> MGGSEVGTVPVTWRLGVDVGERSIGLAAVSYEEDKPKEILAAVSWIHDGGVGDERSGASRLALRGMARRARRLRRFRRARLRDLDMLLSELGWTPLPDKNVSPVDAWLARKRLAEEYVVDETERRRLLGYAVSHMARHRGWRNPWTTIKDLKNLPQPSDSWERTRESLEARYSVSLEPGTVGQWAGYLLQRAPGIRLNPTQQSAGRRAELSNATAFETRLRQEDVLWELRCIADVQGLPEDVVSNVIDAVFCQKRPSVPAERIGRDPLDPSQLRASRACLEFQEYRIVAAVANLRIRDGSGSRPLSLEERNAVIEALLAQTERSLTWSDIALEILKLPNESDLTSVPEEDGPSSLAYSQFAPFDETSARIAEFIAKNRRKIPTFAQWWQEQDRTSRSDLVAALADNSIAGEEEQELLVHLPDAELEALEGLALPSGRVAYSRLTLSGLTRVMRDDGVDVHNARKTCFGVDDNWRPPLPALHEATGHPVVDRNLAILRKFLSSATMRWGPPQSIVVELGGGSAGGYAAVALRDRLLSYGEKNGVAQVAVFRGGVTAEARRWLDISIERLFSRVAIFAQSTSTKRLDRRHHAVDAVVLTTLTPGVAKTLADARSRRVSAEFWRRPSDVNRHSTEEPQSPAYRQWKESCSGLGDLLISTAARDSIAVAAPLRLRPTGALHEETLRAFSEHTVGAAWKGAELRRIVEPEVYAAFLALTDPGGRFLKVSPSEDVLPADENRHIVLSDRVLGPRDRVKLFPDDRGSIRVRGGAAYIASFHHARVFRWGSSHSPSFALLRVSLADLAVAGLLRDGVDVFTAELPPWTPAWRYASIALVKAVESGDAKQVGWLVPGDELDFGPEGVTTAAGDLSMFLKYFPERHWVVTGFEDDKRINLKPAFLSAEQAEVLRTERSDRPDTLTEAGEILAQFFPRCWRATVAKVLCHPGLTVIRRTALGQPRWRRGHLPYSWRPWSADPWSGGTPHHHHHH

Here we further characterized the PAM recognized by AceCas9 and report crystal structures of AceCas9 without its HNH domain (AceCas9–ΔHNH) bound with a guide RNA and DNA targets. Similar to other Cas9, AceCas9 contains the conserved RuvC domain that is connected by the arginine-rich bridge helix (BH) to the nucleic acid recognition domain (REC) and the PAM-interacting domain (PID). Unlike other Cas9, AceCas9 functions at an elevated temperature, interacts with its specific RNA partner, and recognizes the unique 5′-NNNCC-3′ PAM. We show that AceCas9 contacts the 5′-NNNCC-3′ PAM by forming a network of hydrogen bonds with both the cytosine and guanine bases.

Finally, to directly observe the impact of PAM sequence on AceCas9 interactions, we co-crystalized AceCas9, sgRNA94, and a DNA target containing the 5′-NNNTC-3′ PAM, or C4*T mutant, under a nearly identical condition as that of the wild-type complex. The C4*T (TC PAM) crystal diffracted to 3.61 Å and has a shorter b-axis than that of the wild-type complex crystal (112 versus 119 Å), indicating a structural change in the complex. While a non-PAM sequence in a dsDNA likely prevents unwinding and subsequent formation of the R-loop, the artificially constructed C4*T oligos lacking the paired protospacer helix in our co-crystallization studies are attached to AceCas9 RNP largely via the guide-TS heteroduplex, which allowed us to examine how the TC PAM may interact with AceCas9 PID. Superimposing of the refined C4*T to that of the wild-type complex structure revealed rotations of both the PAM DNA helix and the REC2 domain toward each other. As a result, the three residues that contact the PAM in the wild-type complex shifted up to 5.5 Å away from the 5′-NNNTC-3′ PAM. We infer that should AceCas9 encounters a dsDNA with the TC PAM, it would have a weak interaction with TC, thus preventing local unwinding and cleavage of the dsDNA substrate. Mutation of the 5′-NNNCC-3′ to 5′-NNNTC-3′ severely impaired AceCas9 activity and destabilized the AceCas9–PAM interaction.>SNAGGSSPITGLVYDQRMMLHHNMWDSHHPELPQRISRIFSRHEELRLLSRCHRIPARLATEEELALCHSSKHISIIKSSEHMKPRDLNRLGDEYNSIFISNESYTCALLAAGSCFNSAQAILTGQVRNAVAIVRPPGHHAEKDTACGFCFFNTAALTARYAQSITRESLRVLIVDWDVHHGNGTQHIFEEDDSVLYISLHRYEDGAFFPNSEDANYDKVGLGKGRGYNVNIPWNGGKMGDPEYMAAFHHLVMPIAREFAPELVLVSAGFDAARGDPLGGFQVTPEGYAHLTHQLMSLAAGRVLIILEGGYNLTSISESMSMCTSMLLGDSPPSLDHLTPLKTSATVSINNVLRAHAPFWSSLR[2x]

Histone deacetylases (HDACs) regulate the acetylation state of lysine residues of histones as well as other protein substrates, and therefore play a pivotal role in many cellular processes. Specifically targeting two or more distinct HDACs can also be beneficial, but this presents a particular challenge when those two HDACs belong to different isozyme classes with different structural requirements for efficient binding (the Zn2+‐dependent HDACs are grouped into Class I (HDACs 1,2,3,8), Class IIa (HDACs 4,5,7,9), Class IIb (HDACs 6,10) and Class IV (HDAC11)). We report the synthesis and evaluation of a class of selective multitarget agents for the inhibition of HDAC6, HDAC8, and HDAC10. Hybridization of the two inhibitor structures resulted in dihydroxamic acids with benzyl‐indole and ‐indazole core motifs.

The structure of this complex reveals that 3a binds to HDAC6 as a single conformer. The catalytic Zn2+ ion is coordinated in monodentate fashion by the hydroxamate N−O− group of 3a (average O−Zn2+ separation=2.1 Å), and the hydroxamate C=O group accepts a hydrogen bond from the Zn2+‐bound water molecule (average O−O separation=2.4 Å). The Zn2+ coordination geometry is similar to that observed for the major conformer of 3a bound to HDAC10. Also similar to the HDAC10‐3a complex, the aromatic ring of the phenylhydroxamate nestles in an aromatic crevice, here defined by F583 and F643. Interestingly, superposition of the two enzyme‐inhibitor complexes reveals that the capping group conformation of 3a differs between the HDAC6 and HDAC10 complexes. As observed in the HDAC10‐3a complex, the capping group is clamped down by E24 of the P23(E,A)CE motif; however, the capping group of 3a in the HDAC6 complex is oriented toward solution; the indole hydroxamate makes hydrogen bond interactions with N645 as well as R788 of a symmetry mate in the crystal lattice. Since the inhibitor capping group has a specific binding site in a pocket in the active site of HDAC10 that is not conserved in the active site of HDAC6, this feature must contribute to selectivity for binding to HDAC10.> MMVISEKVRKALNDQLNREIYSSYLYLSMATYFDAEGFKGFAHWMKKQAQEELTH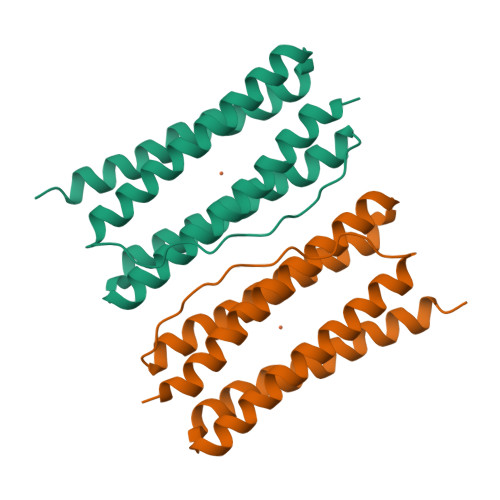AMKFYEYIYERGGRVELEAIEKPPSNWNGIKDAFEAALKHEEFVTQSIYNILELAYEEKDHATVSFLKWFVDEQVEEEDQVREILDLLEKANG> XVDKV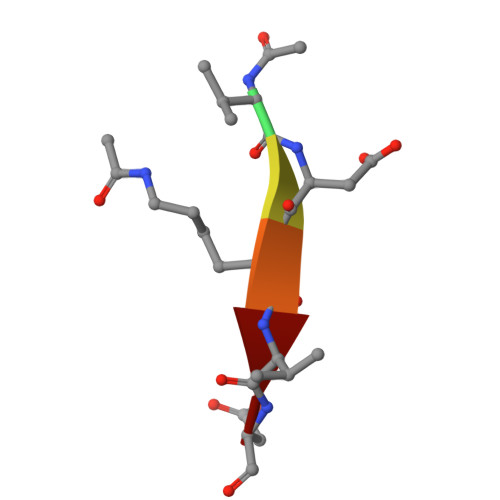D> GILDPEERYEHQLRQLNDMGFFDFDRNVAALRRSGGSVQG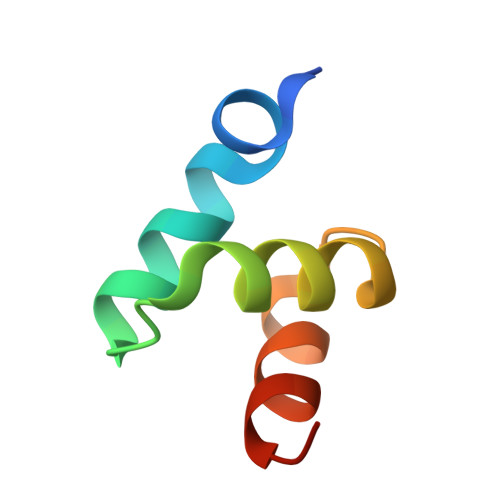ALDSLLNGDV> MVIDSKQDLPQYTKDSGSESDSDSSNNFIVESPSIPSSKSATVVLNSEEYEDDEGDDLNGLDAELIDNITYEGDEDETMFVGLKEKQKLHLSGVFRLQVVKGGIVYNNVHYNASREILTFWHPLSQSIPTIDFSHFAGWQDTFFMPRNNRFKIRD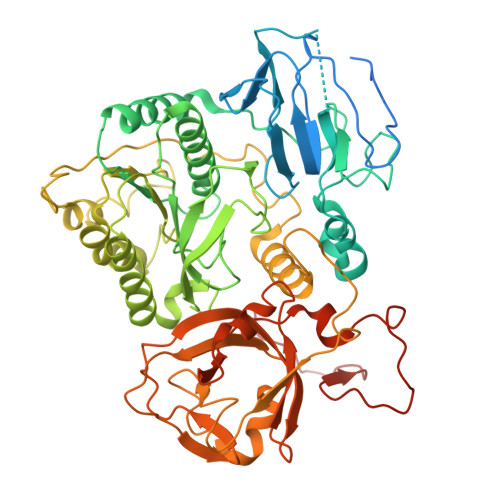EEFKSFPCVLRVFNSNHTGLLEAGHLYRDVNYLWKPKEPYFPLNERTTYHLLHESDRIQSLSVPGYWSTPLEKLYLSHKNAAYDTRIMVIGGKNSGKSTFLRLLLEKFTQDIRDSTTSQEELVYLDLDPGQPEYSLPDSISLNKILSSPISLGQHLCQGSNFQTLLQFYAGSSSPQDEPTSYLNCADKLIDHLEEQAFFGTSLLNLPGWIKGFGMQILNHIIRKYKPTHLLFLETANSKRHLDELTIPQSFSTSLRDAYAPEVVRVPAHSLNHTLSSRFHASQLRTFKILALFHKITQFDYDFAPLLKSAPLQISYGKGKSGIKGIQFPMEFQDLNPQDIKSALEGTVIGIYTYSGEDSLEVKSLNTFPILQSCTSSSKNFITLGLIHSIDTSQQIMNIYVPPCHTQILDKQPEDAQWIIVRNKTETPFCDFLPSPRTITWDDNIQIPFATFERRKKLEHVWKVRKNVMRRGQFMKR> AQTLCDQYATYSNGRYT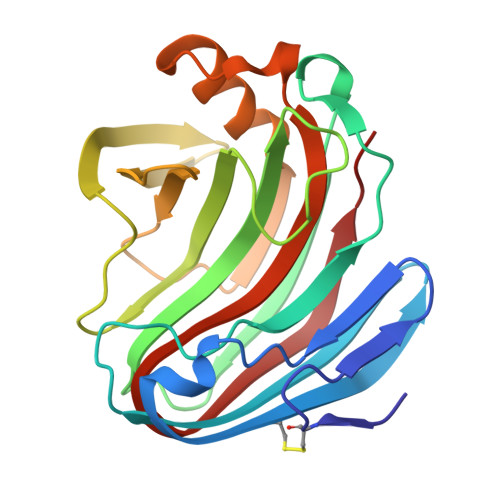VNNNLWGKSSGSGSQCTYVDSISNSGVAWHTTWTWSGGDNQVKSYANSQVSLTKKLVSQISSIPTTVQWSYDNTNTRADVAYDLFTAADINHVTYSGDYELMIWLARYGSVQPIGSQIDSVNIGGHTWELWYGGSTQKTYSFVSATPITSFSGDVMDFWDYLTSRHGYPASSQYLINMQFGTEPFTGGPATLRVSQWTASVN> MHNHNHNHNHNHNGGENLYFQGASLTEIEHLVQSVCKSYRETCQLRLEDLLRQRSNIFSREEVTGYQRKSMWEMWERCAHHLTEAIQYVVEFAKRLSGFMELCQNDQ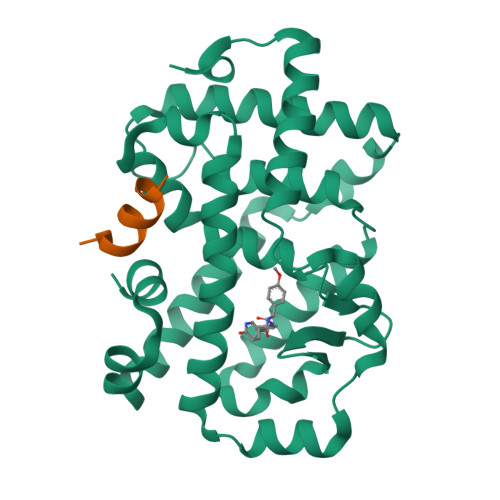IVLLKAGAMEVVLVRMCRAYNADNRTVFFEGKYGGMELFRALGCSELISSIFDFSHSLSALHFSEDEIALYTALVLINAHRPGLQEKRKVEQLQYNLELAFHHHLCKTHRQSILAKLPPKGKLRSLCSQHVERLQIFQHLHPIVVQAAFPPLYKELFSGGGKEKHKILHRLLQDSS;> KEKHKILHRLLQDSS(3S,6S)-3-(4-hydroxybenzyl)-6-(1H-indol-3-ylmethyl)piperazine-2,5-dione | 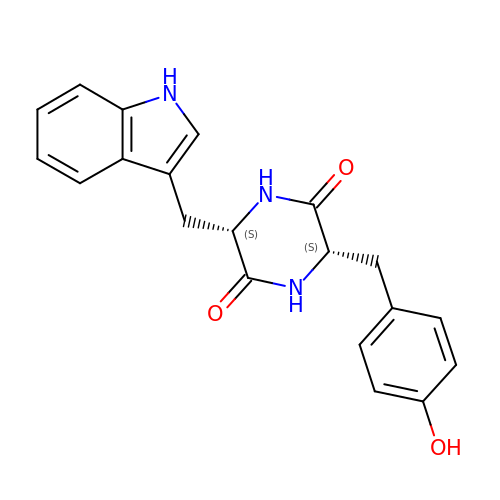C20 H19 N3 O3 | ZJDMXAAEAVGGSK-ROUUACIJSA-N> CIKGNVDLVFLFDGSM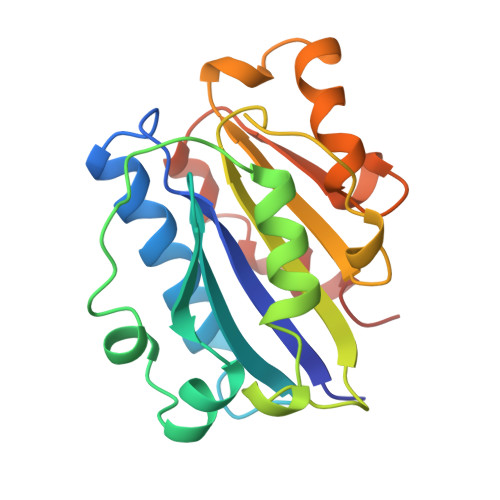SLQPDEFQKILDFMKDVMKKLSNTSYQFAAVQFSTSYKTEFDFSDYVKRKDPDALLKHVKHMLLLTNTFGAINYVATEVFREELGARPDATKVLIIITDGEATDSGNIDAAKDIIRYIIGIGKHFQTKESQETLHKFASKPASEFVKILDTFEKLKDLFTELQKKIYVIEG>MGQGDESERIVINVGGTRHQTHRSTLRTLPGTRLAWLAEPDAHSHFDYDPRADEFFFDRHPGVFAHILNYYRTGKLHCPADVCGPLYEEELAFWGIDETDVEPCCWMTYRQHRDAEEALDSFGGAPLDNSADDADADGPGDSGDGEDELEMTKRLALSDSPDGRPGGFWRRWQPRIWALFEDPYSSRYARYVAFASLFFILVSITTFCLETHERFNPIVNKTEIENVRNGTQVRYYREAETEAFLTYIEGVCVVWFTFEFLMRVIFCPNKVEFIKNSLNIIDFVAILPFYLEVGLSGLSSKAAKDVLGFLRVVRFVRILRIFKLTRHFVGLRVLGHTLRASTNEFLLLIIFLALGVLIFATMIYYAERIGAQPNDPSASEHTHFKNIPIGFWWAVVTMTTLGYGDMYPQTWSGMLVGALCALAGVLTIAMPVPVIVNNFGMYYSLAMAKQKLPKKKKKHIPRPPQLGSPNYCKSVVNSPHHSTQSDTCPLAQEEILEINRAGRKPLRGMSIAENLYFQ[8x]

Voltage-gated K+ channels of the Kv3 family represent an important subfamily among the 70 different Kv channel genes in the human genome, with specialized biophysical properties to sustain high-frequency firing of action potentials. The combination of ultra-fast activation and deactivation kinetics and high activation potential of these channels are key for their ability to repolarize the membrane and terminate the action potential. Like other pore-forming subunits of Kv channels, Kv3 members are comprised of an N-terminal cytoplasmic T1 domain, which is involved but not required for Zn2+-mediated tetramerization, followed by the voltage-sensing domain (VSD) with transmembrane helices S1–S4 which is connected via a helical linker (S4/S5L) to the pore forming domain (PD) of the channel. Here, we present cryo-EM structures of the human Kv3.1a channel in an activated state, providing mechanistic insights into the modulation of Kv3 channels by the cytoplasmic T1 domain.

To elucidate the structural determinants underlying the biophysical properties of Kv3 channels, we purified the shorter α-isoform of Kv3.1 from mammalian cells and determined cryo-EM structures under different sample conditions (apo, Zn2+-containing vs. Zn2+-free). We achieved 3D reconstructions between 3.1 and 3.5 Å for the different conditions, which show only minor differences in the overall structure, and no clear densities for additional Zn2+ sites other than the known sites in the T1 domain16 (see Supplementary discussion). The polar head group of the lipid is stabilized by interactions with the imidazole group of H212 in the S1/S2 linker and backbone interactions with Q409 and M414 in S6. Our maps also show densities in the selectivity filter which likely correspond to K+ ions from the purification buffer.>GECGDMFNGDDSSVVRRSANYPANLWDYDFLQSLGRHSSVTEEHVGLAEKLKGEVKSLITGPMEPLAKLEFIDSVRRLGLKYQFETEMKEALANISKDGYDSWWVDNLRATALRFRLLRENGIFVPQDVFERFQNKETGKFKNELCEDVKKLLNLYEASFLGWEGEDILDEARTFSTAQLKNVEKKISSPNLAKIVHHALDLPLHWRAIRYEARWFIDIYEDEEDMNPTLLKYAKLDFNIVQSFHQAEIGRLARWWVGTGLDKLPFARNGLIQSYMYAIGMLFEPH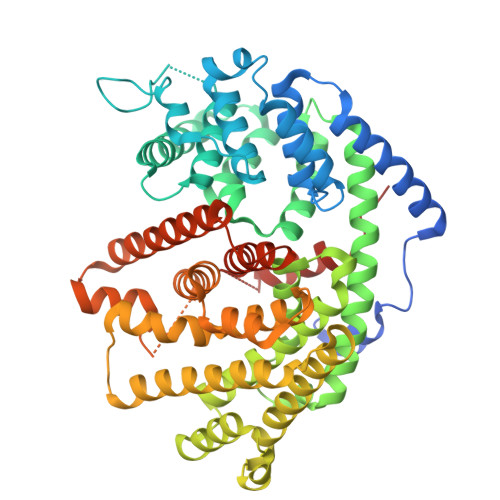LGEVREMEAKVGALITTIDDVYDVYGTMEELELFTDITERWDINRVDQLPRNIRMPLLTMFNTSNDIGYWALKERGFNGIPYTAKVWADQLKSYTKEAKWFHEGHKPTLEEYLENALVSIANPNLLVTSYLLTVDNPTKEKLDYVDSLPLFVRASCILCRIINDLGTSPDEMERGDNLKSIQCYMNETGASQEVAREHIEGLVRMWWKRLNKCLFEPSPFTEPFLSFTINVVRGSHFFYQYGDGYGNAESWTKNQGMSVLIHPITLDEE[2x]>NNLQNIIYNPVIPFVGTIPDQLDPGTLIVIRGHVPSDADRFQVDLQNGSSMKPRADVAFHFNPRFKRAGCIVCNTLINEKWGREEITYDTPFKREK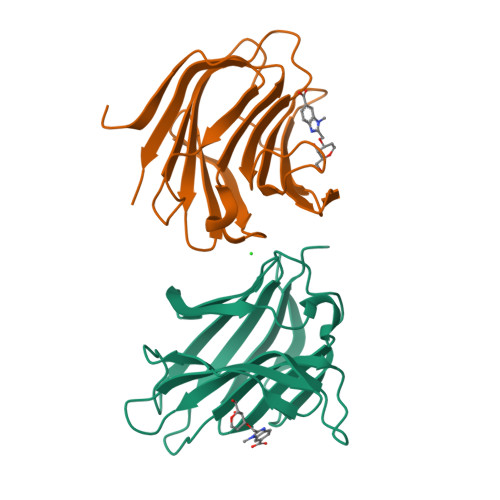SFEIVIMVLKDKFQVAVNGKHTLLYGHRIGPEKIDTLGIYGKVNIHSIGFSFSSD[2x]>[2x]MSELEKAVVAL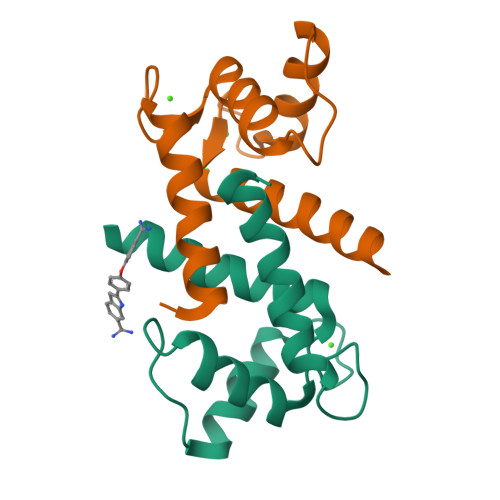IDVFHQYSGREGDKHKLKKSELKELINNELSHFLEEIKEQEVVDKVMETLDSDGDGECDFQEFMAFVAMITTACHEFFEHE Indanomycin is an antibiotic from the pyrroloketo­indane family which is known to act as an effective ionophoric agent against Gram-positive bacteria. IdmH is a homodimer, with the individual protomers consisting of an α+β barrel. Each protomer contains a deep hydrophobic pocket which is proposed to constitute the active site of the enzyme.

To improve crystallization, a number of variants were produced to reduce the surface entropy or to truncate predicted surface loops (Roy et al., 2010). One variant, containing a deletion of residues 99–107, resulted in large, easily reproducible crystals in the cubic space group F23 [Supplementary Fig. S5(b)] from new crystallization conditions. The asymmetric unit comprises one copy of the IdmH-Δ99–107 dimer with the entire polypeptide chain successfully modelled into density, except for the N- and C-terminal regions. Both the selenomethionine-labelled protein structure and the isomorphous native structure of IdmH-Δ99–107 were modelled independently, giving almost identical structures that superpose with an r.m.s.d. of 0.12 Å over 257 amino acids. The remainder of the structural description will focus on the unlabelled native protein as this should best represent the natural form of the enzyme. With this structure in hand, the crystal structure of wild-type IdmH was determined by molecular replacement using a single subunit of IdmH-Δ99–107 as a search model.

>[2x]GSHMAHQPSDTIAGLYEAFNSGDLETLRELIAPDAVIHLPGTAGDAEHPPGTPRDREGWLGVWQFTQAFFPDMTATVQDIVQTGDLVATRCVARGTHSGRPFEMTMLNMSRVRDGRIVEHWTISDNVTMLAQLGVKASL> MSNIEHGLSFIDIMVFAIYVAIIIGVGLWVSRDKKGTQKSTEDYFLAGKSLPWWAVGASLIAANISAEQFIGMSGSGYSIGLAIASYEWMSAITLIIVGKYFLPIFIEKGIYTIPEFVEKRFNKKLKTILAVFWISLYIFV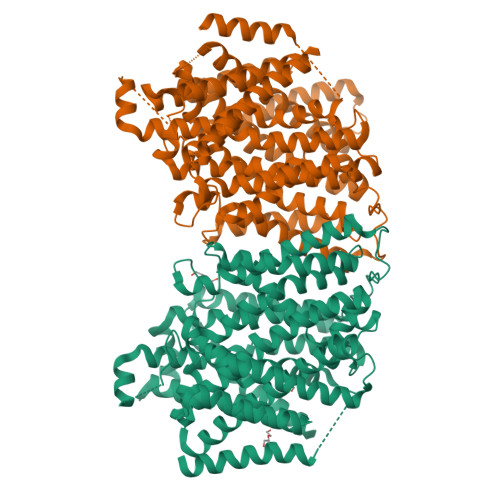NLTSVLYLGGLALETILGIPLMYSILGLALFALVYSIYGGLSAVVWTDVIQVFFLVLGGFMTTYMAVSFIGGTDGWFAGVSKMVDAAPGHFEMILDQSNPQYMNLPGIAVLIGGLWVANLYYWGFNQYIIQRTLAAKSVSEAQKGIVFAAFLALIVPFLVVLPGIAAYVITSDPQLMASLGDIAATNLPSAANADKAYPWLTQFLPVGVKGVVFAALAAAIVSSLASMLNSTATIFTMDIYKEYISPDSGDHKLVNVGRTAAVVALIIAALIAPMLGGIGQCFQYIQEYTGLVSPGILAVFLLGLFWKKTTSKGAIIGVVASIPFALFLKFMPLSMPFMDQMLYTLLFTMVVIAFTSLSTSINDDDPKGISVTSSMFVTDRSFNIAAYGIMIVLAVLYTLFWVNADAEITLIIFGVMAGVIGTILLISYGIKKLIKASYKSGGSPGHHHHHH;> XXXXXXXXXXXXXXXXXXXXXXXXXXXXXXXXXXXXXXXXXXXXXXXXXXLPWWAVGASLIAANISAEQFIGMSGSGYSIGLAIASYEWMSAITLIIVGKYFLPIFIEKGIYTIPEFVEKRFNKKLKTILAVFWISLYIFVNLTSVLYLGGLALETILGIPLMYSILGLALFALVYSIYGGLSAVVWTDVIQVFFLVLGGFMTTYMAVSFIGGTDGWFAGVSKMVDAAPGHFEMILDQSNPQYMNLPGIAVLIGGLWVANLYYWGFNQYIIQRTLAAKSVSEAQKGIVFAAFLALIVPFLVVLPGIAAYVITSDPQLMASLGDIAATNLPSAANADKAYPWLTQFLPVGVKGVVFAALAAAIVSSLASMLNSTATIFTMDIYKEYISPDSGDHKLVNVGRTAAVVALIIAALIAPMLGGIGQCFQYIQEYTGLVSPGILAVFLLGLFWKKTTSKGAIIGVVASIPFALFLKFMPLSMPFMDQMLYTLLFTMVVIAFTSLSTSINDDDPKGISVTSSMFVTDRSFNIAAYGIMIVLAVLYTLFWVNADAEITLIIFGVMAGVIGTILLISYGIKKLIKASYKSGGSPGHHHHHH>[4x]GSGMEKVQMAKEEELAESSAISAKEAKIEDTRDKIQALDESVDELQQVLLVTSEELEKLEGRKEVLKERKKNAVQNQEQLEEAIVQFQQKETVLKEELSKQEAVFETLQAEVKQLRAQVKEKQQALSLHNENVEEKIESGGSGGSRLTKQKQTQSS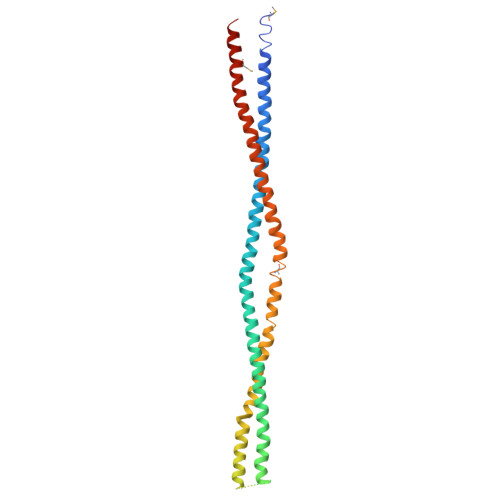TKESLSNELTELKIAAAKKEQACKGEEDNLARLKKELTETELALKEAKEDLSFLTSEMSSSTSGEEKLEEAAKHKLNDKTKTIELIALRRDQRIKLQHGLDTYERELKEMKRLYKQKTTLLKDEEV> APEKGK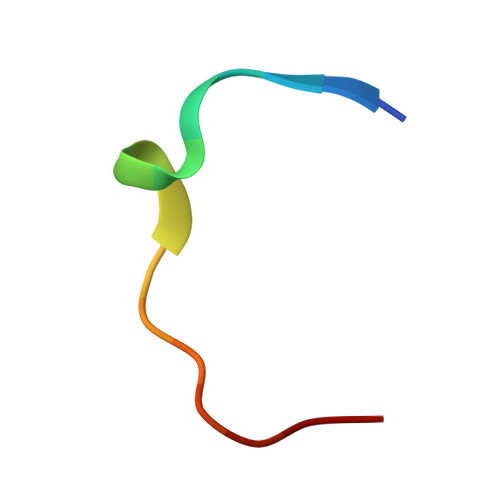YTKEVNFFDE>MAHHHHHHSSGLEVLFQGPNTPVLEKNNVTLTGGGENVTKELKDKFTSGDFTVVIKYNQSSEKGLQALFGISNSKPGQQNSYVDVFLRDNGELGMEARDTSSNKNNLVSRPASVWGKYKQEAVTNTVAVVADSVKKTYSLYANGTKVVEKKVDNFLNIKDIKGIDYYMLGGVKRAGKTAFGFNGTLENIKFFNSALDEETVKKMTTNAVTGHLIYTANDTTGSNYFRIPVLYTFSNGRVFSSIDARYGGTHDFLNKINIATSYSDDNGKTWTKPKLTLAFDDFAPVPLEWPREVGGRDLQISGGATYIDSVIVEKKNKQVLMFADVMPAGVSFREATRKDSGYKQIDGNYYLKLRKQGDTDYNYTIRENGTVYDDRTNRPTEFSVDKNFGIKQNGNYLTVEQYSVSFENNKKTEYRNGTKVHMNIFYKDALFKVVPTNYIAYISSNDHGESWSAPTLLPPIMGLNRNAPYLGPGRGIIESSTGRILIPSYTGKESAFIYSDDNGASWKVKVVPLPSSWSAEAQFVELSPGVIQAYMRTNNGKIAYLTSKDAGTTWSAPEYLKFVSNPSYGTQLSIINYSQLIDGKKAVIL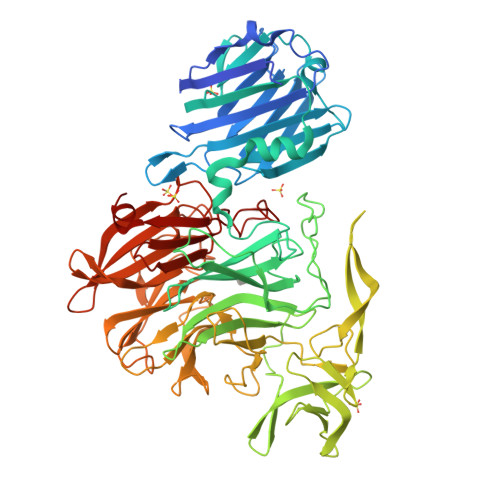STPNSTNGRKHGQIWIGLINDDNTIDWRYHHDVDYSNYGYSYSTLTELPNHEIGLMFEKFDSWSRNELHMKNVVPYITFKIEDLKKN[2x]>MGHHHHHHEDRDPTQFEERHLKFLQQLGKGNFGSVEMCRYDPLQDNTGEVVAVKKLQHSTEEHLRDFEREIEILKSLQHDNIVKYKGVCYSAGRRNLKLIMEYLPYGSLRDYLQKHKERIDHIKLLQYTSQICKGMEYLGTKRYIHRDLA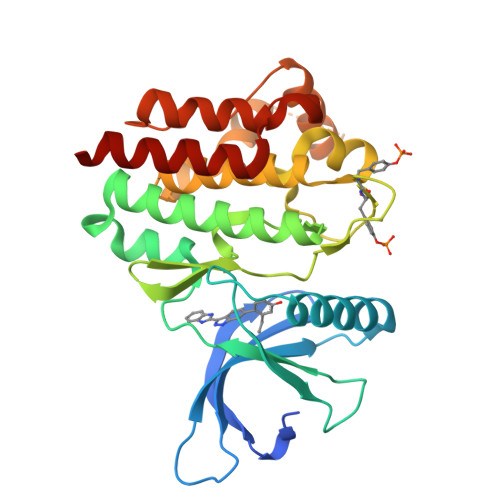TRNILVENENRVKIGDFGLTKVLPQDKEYYKVKEPGESPIFWYAPESLTESKFSVASDVWSFGVVLYELFTYIEKSKSPPAEFMRMIGNDKQGQSIVTHLIELLKNNGRLPRPDGCPDEIYMIMTECWNNNVNQRPSFRDLALRVDQVRDNMAG[2x]>[60x]MYFFSVDPRNGASKSGDVCGSCCCESISARPGEVNGVMVSYAAWSAPLRGHGLTNKTTFEIDGVSVTPPKVSNAFGRTKVGVVFEGTLSDLFPNPEGEQVEYEISELNGPSNGVVELGANGAFTYTPGALFTGVDRFWFSINGNIGEYVISVDPTTSELPQPPFTTPVYVPAARRSVDPRTHVLKFVLGVSPAAIPGDVYRLTVRQVAIDCDGNEFVHISCYDISIGSCG;>MLGIPLLTRKAALTPPAPSANPAKIFIRRFFSAGVAKNVVSYSNVMAAQRAMEHPVAFRCLDKLGLTVQSVKWDVGKDPQNTQVGDGGMSASQRKALQQILQRPNPTMSGAQLRYSAALSWACFGRMAFKVSVMSDGSVNAIWPLGIPFLKQKFDRYGDVESFQYGDEAGKETIPSFTKVEKNDK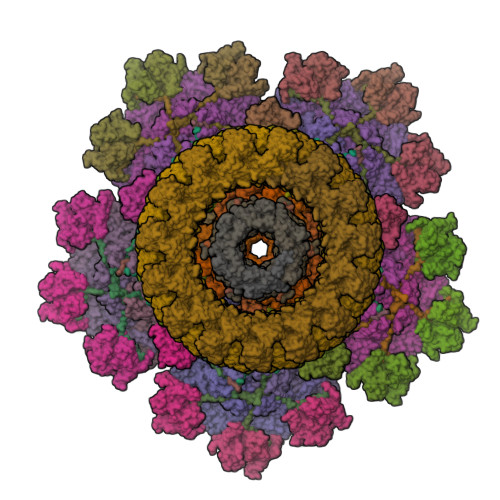GRPIKNYAFMIVKPSINGAMNFDVQNTPLQAIGVPVALYDALMARAIDSADGTPNSKWLVTASRDLDDGQAKEVKEGIEETKPGGDNGGEIIFIAGTDVKVQEMKNDLSDIHSKVPLDDQARTIAGNFGIPIALLGFAGADGSKFANNYDESRKAFFEDTIEPGYLTPLEDGFSMFLCGAGYRVIFDRDSIPALRKSRADIAATYDKVTFITEEEKREVTGWPAKKEGQTQNDDA[12x];>MRTADRKHRVIVCSQQSDVDDEGRLLITRAGVIQGWAAIAPVKAIRFSQDGVSMQKDTMQPTHDITMNYNPDVNVSVSAWVYEHRLKSPPRWFKVLSVVNVDECSRYMKIRCRLVETSDDVTPPVEEEKNSFGAVKIDIPL[6x];>METKLTYGNRVTLPEFAKYIVAPAFHEIEGRAIPVTGVDDDASGTQATKLPFVLVGLRQGDTSGPATIAGNSTINLRDDFIVEFNMKKERYRDRKGGETPFFSYYDYESIRDRLFNSMIEFSGEHGITFEFVSLDISTEGDVVYIEFRFRQNYEWCETVREADTTIEAGRFSINLQGC[6x];>MACNKQNGVKNILITFTDCDTQEVIGPISHEQPDDTLPTYKNCAWTNTALTNGYVQRSASNATMTLPVVRDLRVPLAFYQGCAQVDVQVEKFDGTVMTLTEGAVVEPEESDGRSVTMNIVASEIDELLPPGSLAAA[6x];>MNLDTLLPLQTIREHAKCDDNPRVTDDLLKLYREAAFEAAELYTGLSFTPEKTIVEPIRLKGRRGKIILSATPIAGRPVVFYGGGLGSPLELIPRPGSNVLFFPYGSPDRFQTWGDCHTCDVESQLMATYVTGRRCENSVPAGIIIGILKLIAWNINNPGDEVMSVRNTLNANAQGLIGGTNNGAVISGAQDEWFRYRRVLL[12x];>[25x]MVKLNCRPLCQAPTASRLVSPPCFICRGVAPSAPVTPG;>MDCRNLCGAAAPSRLVQPGCFICRGVAVSIPPAAPGPATSVFDTPPSTFSLRPDGTIIAGTGIRGDHASVGTDGTIEMFIVPFIGDVTGSELTHPYAVELQDGEELAIAFGVTLKSGYGARITEYYDVSLFLENGGNSKELTLQPANTKSGYVWSDGHGYNITDSDGDLHTVQNVTRPVWFEMTEPGIVGVIMEARYKATGLVSSSISITVNVTYAD[5x];>MANKESELNGLDDIHSDIEKLSAHVEKFSDGMDEKYKELTARFDGVKGDNDAIRKAVADATKEYAELSAKHQFFTEELAAMKARLDTPIMRSQAELDDHDRKTAIQLQRNMHEFRGGDPKEFVADESNLVDLKAYRSAVRKMLKVGIESKERVIASMTDVERKAFEASTIGPAFFTPQVLALEVDCNIECASLLDLYGQIEVSRSTFTYMKIADYGQLGEYTCDAKCDAEFGEPGNIRHLEGKTYDYRGVFCFNRKNLQEANYDFLSFMIGAAQRSHRINRNQALMIGKGVNEPKGWLTENCFPVFQTLPVDVNGTSTPAFLAQDWRRFVTSFPAEYGEARSVMHQNVFGYLAAMVDANGRFLFGDGDLTFTPDLVRERIRISNCLPDPTEGNTKGGTGQDAFAAGSFVAAQAAWKTAFYAVEKRPMFFEQYEGGSSAWCVKYQFGAEDGGFVGCCEHGRILQIG[30x];>[40x]MNFNVGVDFPSFIAWDGEESFPVKVDGFNQFGFTFKTIAALTAATTFNIFYHEPSDADPCVPGPAIRVPEVPFCDTVLLSEDGLAAVTLPETVTPDSFCAGTVPCMNGQWISIAPATGSETNAANVQITVTMKGATR> MRDRVRWRVLSLPPLAQWREVMAALEVGPEAALAYWHRGFRRKEDLDPPLALLPLKGLREAAALLEEALRQGKRIRVHGDYDADGLTGTAILVRGLAALGADVHPFIPHRLEE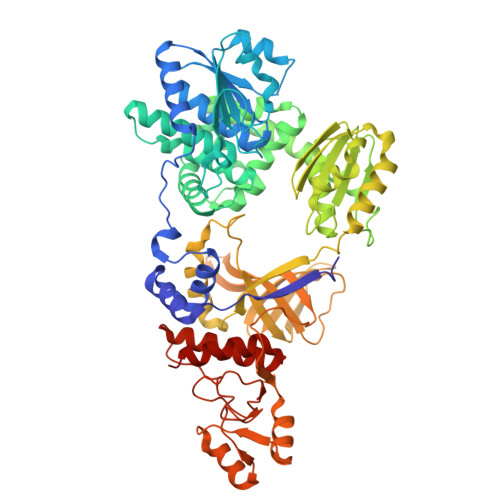GYGVLMERVPEHLEASDLFLTVDCGITNHAELRELLENGVEVIVTDHHTPGKTPPPGLVVHPALTPDLKEKPTGAGVAFLLLWALHERLGLPPPLEYADLAAVGTIADVAPLWGWNRALVKEGLARIPASSWVGLRLLAEAVGYTGKAVEVAFRIAPRINAASRLGEAEKALRLLLTDDAAEAQALVGELHRLNARRQTLEEAMLRKLLPQADPEAKAIVLLDPEGHPGVMGIVASRILEATLRPVFLVAQGKGTVRSLAPISAVEALRSAEDLLLRYGGHKEAAGFAMDEALFPAFKARVEAYAARFPDPVREVALLDLLPEPGLLPQVFRELALLEPYGEGNPEPLFLLFGAPEEARRLGEGRHLAFRLKGVRVLAWKQGDLALPPEVEVAGLLSENAWNGHLAYEVQAVDLRKPEALEGGIAPFAYPLPLLEALARARLGEGVYVPEDNPEGLDYAWKAGFRLLPPEEAGLWLGLPPRPVLGRRVEVALGREARARLSAPPVLHTPEARLKALVHRRLLFAYERRHPGLFSEALLAYWEVNRVQEPAGSP>MRVLITGCGSRGDTEPLVALAARLRELGADARMCLPPDYVERCAEVGVPMVPVGRAVRAGAREPGELPPGAAEVVTEVVAEWFDKVPAAIEGCDAVVTTGLLPAAVAVRSMAEKLGIPYRYTVLSPDHLPSEQSQAERDMYNQGADRLFGDAVNSHRASIGLPPVEHLYDYGYTDQPWLAADPVLSPLRPTDLGTVQTGAWILPDERPLSAELEAFLAAGSTPVYVGFGSSSRPATADAAKMAIKAVRASGRRIVLSRGWADLVLPDDGADCFVVGEVNLQELFGRVAAAIHHDSAGTTLLAMRAGIPQIVVRRVVDNVVEQAYHADRVAELGVGVAVDGP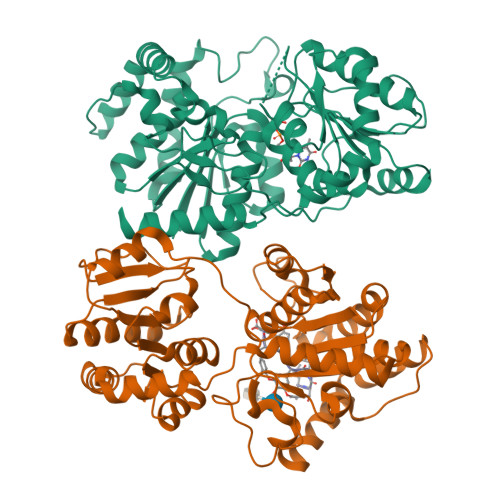VPTIDSLSAALDTALAPEIRARATTVADTIRADGTTVAAQLLFDAVSLEKPTVPALEHHHHHH[2x]>MMSETAPLPSASSALEDKAASAPVVGIIMGSQSDFETMRHADALLTELEIPHETLIVSAHRTPDRLADYARTAAERGLNVIIAGAGGAAHLPGMCAAWTRLPVLGVPVESRALKGMDSLLSIVQMPGGVPVGTLAIGAS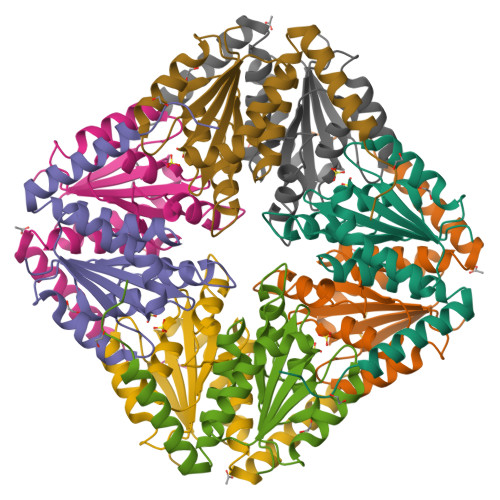GAKNAALLAASILALLNPALAARLETFRALQTASVPNSPITEDK[2x]>[2x]MAHHHHHHMRVEPLTCAIGAELLGVNLADAVHDDGLFAEIRTQLLRHRVLFLRDQDITRAEHVAFARRFGELEDHPVAGSDPEHPGLVRIYKSPDQPNDRYENAWHSDASWRVAPPFGCVLRCIDGPPVGGDTMWANMVLA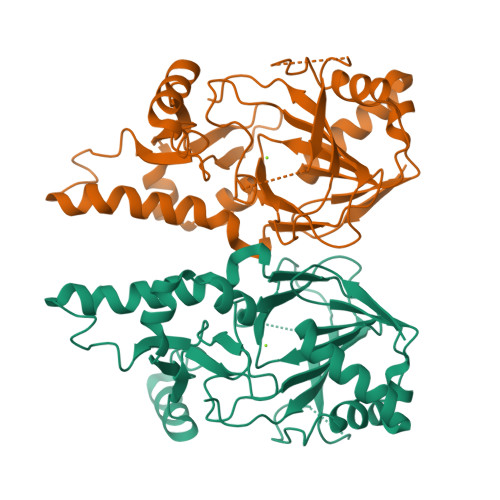YENLPDHVKQQIADLRARHSIEASFGAAMPIDKRLALKAQYPDAEHPVVRTHPETGEKVLYVNAFTTHFTNFHTPARVRVGQDANPGAGQLLHYLIGQAAIPEYQVRWRWKKNSVAIWDNRATQHYAVMDYPPCVRRMERAGIVGDVPF> EVRPFLDVYQRSACQTRETLVSILQEHPDEISDIFRPSCVAVLRCSGCCTDESMKCTPVGKHTADIQIMR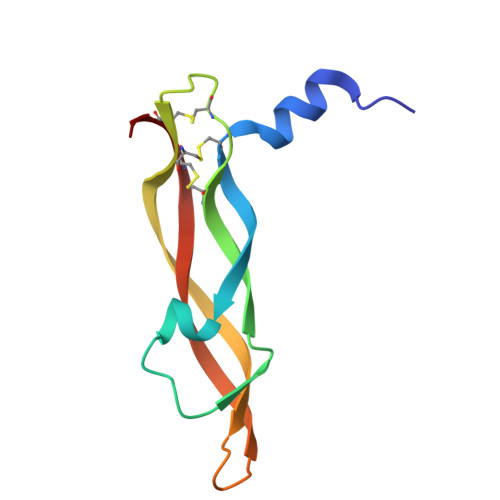MNPRTHSSKMEVMKFMEHTACECRPA>MDNEKGLLIVLSGPSGVGKGTVRKRIFEDPSTSYKYSISMTTRQMREGEVDGVDYFFKTRDAFEALIKDDQFIEYAEYVGNYYGTPVQYVKDTMDEGHDVFLEIEVEGAKQVRKKFPDALFIFLAPPSLEHLRERLVGRGTESDEKIQS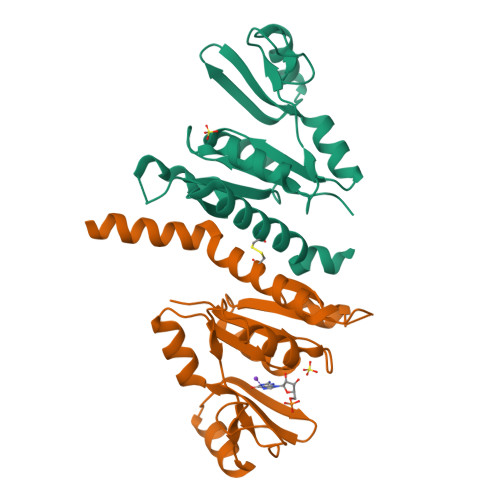RINEARKEVEMMNLYDYVVVNDEVELAKNRIQCIVEAEHLKRERVEAKYRKMILEAKK[4x]>[2x]EAGITGTWYNQLGSTFIVTAGADGALTGTYESAVTATSNEIKRYVLTGRYDSAPATDGSGTALGWTVAWKNNYRNAHSATTWSGQYVGGAEARINTQWLLTSGTTEANAW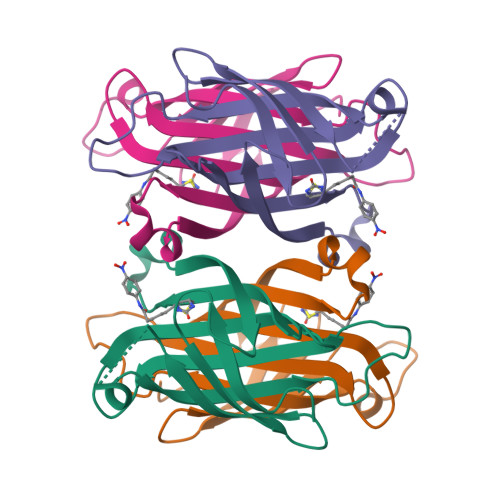KSTRVGHDTFTKVKP> EDIGKITQAIKE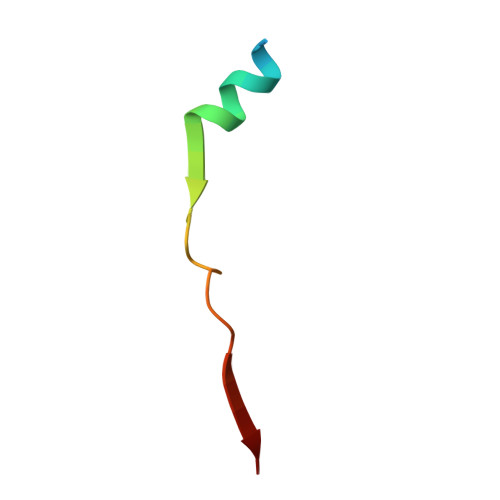CLSKDPGAIDEDPFIIEL The PcrA/UvrD helicase functions in multiple pathways that promote bacterial genome stability including the suppression of conflicts between replication and transcription and facilitating the repair of transcribed DNA. An interesting example is provided by the UvrD helicase (also annotated Helicase II, or PcrA in many Gram positive bacteria including Bacillus subtilis) which has been implicated in nucleotide excision repair (NER), mismatch repair, homologous recombination and rolling circle replication mechanisms. This multi-functionality is reflected in the ability of UvrD/PcrA to interact physically and functionally with many different partner proteins including UvrB, MutL, MutS, RecA and RepC/D. We and others have recently shown that PcrA/UvrD also interacts with RNA polymerase (RNAP), and this interaction could be important for the UvrD-dependent backtracking of stalled RNA polymerase. The extreme C-terminal region of PcrA/UvrD is important for interaction with both RNAP and UvrB. In this report, we define a small folded RNA polymerase interaction domain in Geobacillus stearothermophilus PcrA and have solved its structure at high resolution.

To test this idea, we designed a new shorter version of the PcrA CTD using the homology models as a guide. This construct, which we call PcrA-short Ct (PcrA-sCt), includes residues 673–724 of the native PcrA protein. Crystals of PcrA-sCt (with the histidine tag removed) were obtained using the sitting drop vapor diffusion method. The structure was solved using a heavy atom derivative at a final resolution of 1.5 Å (Rfree = 22.2%). The final model includes all of the residues of the native PcrA sequence (W673 to V724) and an N-terminal glycine from the tag linker region. As predicted, the extreme C-terminal region of PcrA adopts a Tudor-like fold consisting of five anti-parallel beta strands that form a twisted β sheet. It closely resembles other bacterial Tudor domains such as those found in RapA, CarD and Mfd. Interestingly, some key residues that form this aromatic cage appear to be equivalent in PcrA (eg W684, F705). However, PcrA also features a charged lysine residue (K712) in this region. Several highly conserved residues cluster together on the surface of the PcrA Tudor fold that frequently forms a protein:protein interface in other systems. The pulldown assays revealed that each of the single mutant proteins had a severely reduced ability to bind to RNAP.

> PGGGWKVGDRANHRKWGIGTVVSVRGGGDDQELDIAFPSPIGIKRLLAKFAPIEKV>[2x]ADKLFINALKKKFEESPEEKKTTFYTLGGWKQSERKTEFVNAGKEVAAKRGIPQYNPDIGTPLGQRVLMPYQVSTTDT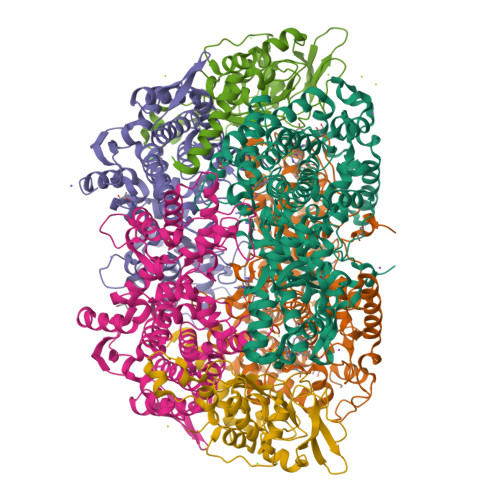YVEGDDLHFVNNAAMQQMWDDIRRTVIVGLNHAHAVIEKRLGKEVTPETITHYLETVNHAMPGAAVVQEHMVETHPALVADSYVKVFTGNDEIADEIDPAFVIDINKQFPEDQAETLKAEVGDGIWQVVRIPTIVSRTCDGATTSRWSAMQIGMSMISAYKQAAGEAATGDFAYAAKHAEVIHMGTYLPVRRARGENEPGGVPFGYLADICQSSRVNYEDPVRVSLDVVATGAMLYDQIWLGSYMSGGVGFTQYATAAYTDNILDDFTYFGKEYVEDKYGLCEAPNNMDTVLDVATEVTFYGLEQYEEYPALLEDQFGGSQRAAVVAAAAGCSTAFATGNAQTGLSGWYLSMYLHKEQHSRLGFYGYDLQDQCGASNVFSIRGDEGLPLELRGPNYPNYAMNVGHQGEYAGISQAPHAARGDAFVFNPLVKIAFADDNLVFDFTNVRGEFAKGALREFEPAGERALITPAK;>AKFEDKVDLYDDRGNLVEEQVPLEALSPLRNPAIKSIVQGIKRTVAVNLEGIENALKTAKVGGPACKIMGRELDLDIVGNAESIAAAAKEMIQVTEDDDTNVELLGGGKRALVQVPSARFDVAAEYSAAPLVTATAFVQAIINEFDVSMYDANMVKAAVLGRYPQSVEYMGANIATMLDIPQKLEGPGYALRNIMVNHVVAATLKNTLQAAALSTILEQTAMFEMGDAVGAFERMHLLGLAYQGMNADNLVFDLVKANGKEGTVGSVIADLVERALEDGVIKVEKELTDYKVYGTDDLAMWNAYAAAGLMAATMVNQGAARAAQGVSSTLLYYNDLIEFETGLPSVDFGKVEGTAVGFSFFSHSIYGGGGPGIFNGNHIVTRHSKGFAIPCVAAAMALDAGTQMFSPEATSGLIKEVFSQVDEFREPLKYVVEAAAEIKNEI[2x];>[2x]AQYYPGTTKVAQNRRNFCNPEYELEKLREISDEDVVKILGHRAPGEEYPSVHPPLEEMDEPEDAIREMVEPIDGAKAGDRVRYIQFTDSMYFAPAQPYVRSRAYLCRYRGADAGTLSGRQIIETRERDLEKISKELLETEFFDPARSGVRGKSVHGHSLRLDEDGMMFDMLRRQIYNKDTGRVEMVKNQIGDELDEPVDLGEPLDEETLMEKTTIYRVDGEAYRDDVEAVEIMQRIHVLRSQGGFNLE>MGSSHHHHHHSSGRENLYFQGHMDKKSLYKYLLLRSTGDMHRAKSPTIMTRVTNNVYLGNYKNAMDAPSSEVKFKYVLNLTMDKYTLPNSNINIIHIPLVDDTTTDISKYFDDVTAFLSKCDQRNEPVLVHCAAGVNRSGAMILAYLMSKNKESLPMLYFLY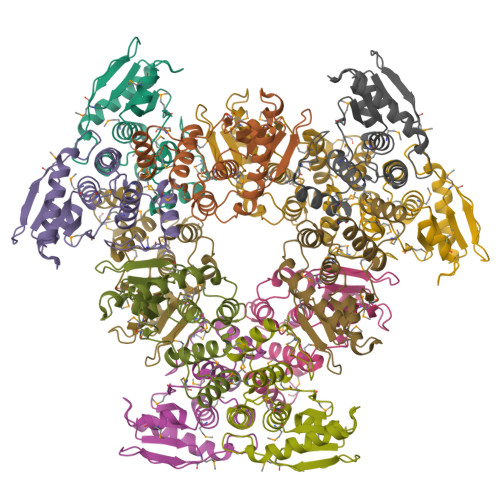VYHSMRDLRGAFVENPSFKRQIIEKYVIDKNGS[4x]First, lipases are very versatile enzymes that catalyze the hydrolysis of ester linkages, primarily in neutral lipids such as triglycerides, which have been extensively characterized and used as CLECs in many studies and from different sources representing an excellent example of a biocatalyst and its applications. Finally, we determined the three-dimensional (3D) models of this commercial lipase crystallized with and without phosphate at 2.0 and 1.7 Å resolutions, respectively. In short, the structure of BioL corresponds to the typical α/β fold highly preserved among different species and has no difference in the catalytic triad composed by Ser146–His258–Asp201 with the nucleophilic Ser146, showing the strained conformation characteristic of the nucleophilic elbow. The structural model presents the closed state of the lid (residue 86–92), as present in many other structural models, which does not prevent the enzymatic activity in the crystals form as shown next.

Initial hits were obtained by the capillary counterdiffusion technique using 0.82 M K/NaH2PO4, 0.1 M Hepes, pH 7.5 (C23 of the CSK screening kit) or 5.0 M sodium formate in 100 mM AcNa pH 7.0 as precipitating agents. Protein and precipitant concentrations were optimized using the batch method while keeping the agarose concentration at 0.1% (w/v). Therefore, the final optimized batch experiments consisted of 500 mL of a protein solution (final concentration of BioL 15 mg·mL–1) in 0.1 M K/NaH2PO4, 0.1 M Tris pH 7.0, and 0.2% (w/v) agarose. Using this condition, we obtained crystals of size ranging from 8 to 20 μm, with 8 ± 2.52 μm being the most abundant at almost 50% of the sample. Interestingly, the only common phosphate-ion moiety among both models did not match their position but appears 2.9 Å apart. Although BioL was crystallized in its closed-lid form, the enzyme was active in water and organic media.

>EVSQDLFNQFNLFAQYSAAAYCGKNNDAPAGTNITCTGNACPEVEKADATFLYSFEDSGVGDVTGFLALDNTNKLIVLSFRGSRSIENWIGNLNFDLKEINDICSGCRGHDGFTSSWRSVADTLRQKVEDAVREHPDYRVVFTGHSLGGALATVAGADLRGNGYDIDVFSYGAPRVGNRAFAEFLTVQTGGTLYRITHTNDIVPRLPPREFGYSHSSPEYWIKSGTLVPVTRNDIVKIEGIDATGGNNQPNIPDIPAHLWYFGLIGTCL[2x]> MENTLGEGSTVNASVDVDQHGNDNNSDSNANAAVAGVANTDTAGEESQQQDESLKDEATVPNTRDAESEAITVTAKQQPTMQANKLDSQETPSTEESRAQNVFGQDNEDSDNLFGETESSVSNNEANTPSIPTNPVDNENNKPAIKEDSTIQDSNGDVKNMEDVKIQKEEEPENNTVIEGVKEESQPDENTKEMDEVEEDDEDDDQPMISPDNSIFGDTKSESKQLGNTSSVANTPSEIPDAHKAEQEDIIEKTESVDKKVDSGEERNEQEREIMNDHSKSANPKKTTITRVEPETFEIPQAHEIVIPSYSKWFNLEKIHSIEVQSLPEFFTNRIPSKTPEVYMRYRNFMVNSYRLNPNEYFSVTTARRNVSGDAAALFRLHKFLTKWGLINYQVDSKLLPKNIEPPL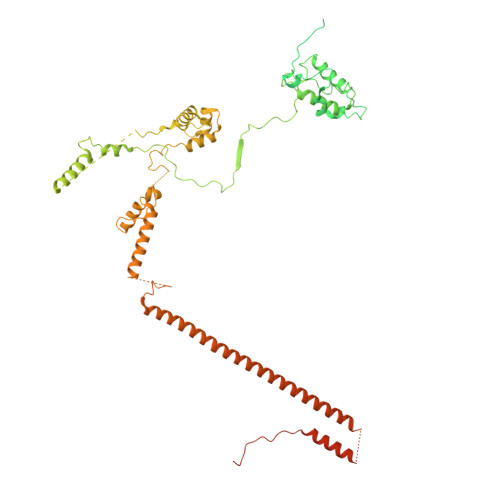TSQYSTRHDAPRGLFPFESYKPSVQLPDMAKLKKMMNTSDSESTLYKYLKESKRKYDEITHPPSTTDDENGDKNDNGGKMNNEVSTSTSMTGDANLLEEGETSRPLKKVKILEQIDENWSKEDLQKLLKGIQEFGADWYKVAKNVGNKSPEQCILRFLQLPIEDKFLYGDGNGKGDNDNGLGPLKYAPHLPFSKSENPVLSTIAFLVGLVNPKTVQSMTQRAIQSAESIKSQKEEISDQKPIEHIKEGSEIAISSLGYRSHIFATNEERQMNFLTNELIRLQMEKLDAKLNHLKKLEKFMELERKTLERQQENLLIQRLNFNQNSSKIVNVLSKCLNLISDSNINNSSVAEKEEIRSQIDHFKSMLSKPETLSIGKNPFNKPNIETGENHNGQSISNENDVKPISIEAPQFYRYWSAGGSGGHHHHHH> MTDSEHVGKTCQIDVLIEEHDERTRAKARLSWAGRQMVGVGLARLDPADEPVAQIGDELAIARALSDLA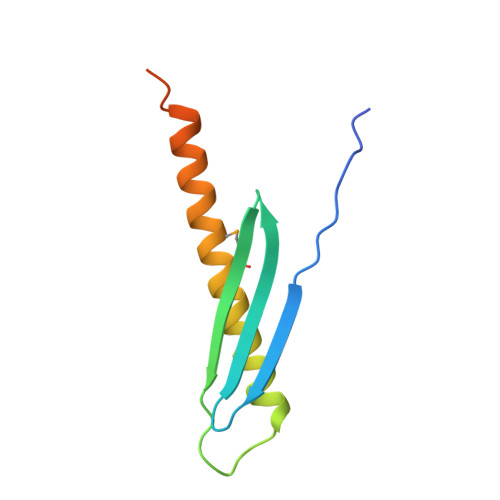NQLFALTSSDIEASTHQPVTGLHHRSHHHHHH> MGMVVALGLDFGASGARAIACDFDSDRSVSVSVTFPKTSQNWPQVWREALWQLLTQIPADWRSRIERIAIDGTSGTVLLCDREGQPQTEPLLYNQACPIDLADLADWVPADHAALSSTSSLAKLWFWQQQFGALPPDWQILAQADWLSLQLHGCSQQSDYHNALKLGYSPDRERFSKNLLDSELGALLPVVHEPGVAIGPILPAIAQEFGLSPDCQICAGTTDSIAAFLASGAHQPGEAVTSLGSTIVLKLLSQVAVSDRLTGVYSHKLGGYWLTGGASNCGGATLRQFFPDTELESLSCQIDPTKKSGLDYYPLPSRGERFPIADPDRLPQLEPRPENPVQFLQGLLEGLTQVETLGYQRLQDLGATPLKRIWTAGGGAKNAVWQQLRQQAIGVPIAIAPNTEAAFGTARLAAFGLAAFHSAGLKRTLEHHHHHH

Synpcc7942_2462 from the cyanobacteria Synechococcus elongatus PCC 7942 encodes a putative sugar kinase (SePSK), and this kinase contains 426 amino acids. The At2g21370 gene product from Arabidopsis thaliana, xylulose kinase-1 (AtXK-1), whose mature form contains 436 amino acids, is located in the chloroplast (ChloroP 1.1 Server). SePSK and AtXK-1 display a sequence identity of 44.9%, and belong to the ribulokinase-like carbohydrate kinases, a sub-family of FGGY family carbohydrate kinases. Domain I exhibits a ribonuclease H-like folding pattern, and is responsible for the substrate binding, while domain II possesses an actin-like ATPase domain that binds cofactor ATP.

Our results suggested that three conserved residues (D8, T11 and D221 of SePSK) play an important role in SePSK function. To identify the function of these three residues of SePSK, we constructed D8A, T11A and D221A mutants. Using enzymatic activity assays, we found that all of these mutants exhibit much lower activity of ATP hydrolysis after adding D-ribulose than that of wild type, indicating the possibility that these three residues are involved in the catalytic process of phosphorylation D-ribulose and are vital for the function of SePSK. Three conserved residues in SePSK were identified to be essential for this function.>GHMSSTNGFGNVYGPSTGTDLFISHSKGVFINGCADCAIYCLPIAGSAFLSNCTNCRVYVACHQLRLKGCTNLDMYVWCASTPIIEECDAMRFGPYRCWVGLLSSCTEDGKTYATHAEWVSRVGEIEDTARTEQNYVKVDDFQWVKKRASPHWCVLAREEERASTTVFGPA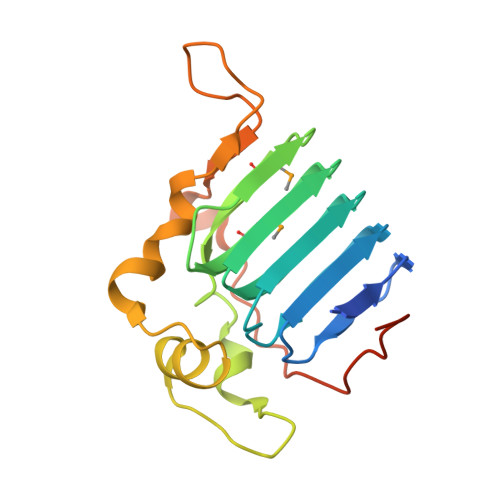TLPSSSTAHSTVAADH[2x]> ETGASYITPYVPMPCMINDTHFLLRGPFEASWAIKLEITDVTTLVVDTDNVANPTNISKCFANNQDERLLGFTMEWFLSGLEHDHHFTPQIICGNVSKGEVNAQVNITMEDHCSQVFLKMRRIFGVFKNPCTSHGKQNVLISVSNWTNQCSGNHLSGTKHHHHHH

The GP1 subunit of the envelope-displayed arenaviral glycoprotein spike complex (GPC) mediates host cell recognition and is an important determinant of cross-species transmission. Maturation of the GPC precursor involves proteolytic cleavage of the polyprotein into a retained and myristoylated stable signal peptide (SSP), a GP1 attachment glycoprotein, and a membrane-anchored GP2 fusion glycoprotein (1–5). We solved the crystal structures of the GP1 glycoproteins from Loei River virus (LORV), an Asiatic rodent-borne OW arenavirus of unknown pathogenicity in humans, and Whitewater Arroyo virus (WWAV), an NW arenavirus associated with spillover into human populations in North America. Both WWAV and LORV GP1s were solved at neutral pH (7.5 to 8.0) and acidic pH (5.6 to 5.0), permitting the first direct analysis of the effect of pH on the structure of GP1 in the absence of cognate GP2.

Crystals of WWAV GP1 were generated under two conditions, buffered to pH 7.5 and 5.6, and X-ray diffraction data were collected to 2.4- and 2.0-Å resolution, respectively. As phase determination by molecular replacement with existing arenaviral GP1 structures failed to yield a solution, the single-wavelength anomalous-dispersion (SAD) method was used for structure elucidation. Crystallographic analysis of WWAV GP1 revealed the characteristic α/β fold that has been observed for other NW arenavirus GP1 structures, as well as in OW arenaviral GP1 glycoproteins in GP2-associated states, comprising a seven-stranded β-sheet with three α-helices positioned on the convex side of the molecule. WWAV GP1 structures determined at both neutral and acidic pHs are nearly identical (0.4-Å root mean square deviation [RMSD]), indicating that exposure to acidic endosomal pH, and subsequent shedding of GP1 from the GPC, is unlikely to induce conformational rearrangements to the molecule. Overlay analysis revealed that while the independently reported WWAV GP1 structures were essentially identical and exhibited an RMSD of 0.9 Å, minor structural differences were observed in loop 5 of the glycoprotein, indicating inherent flexibility in the region or a requirement for the quaternary architecture of the GPC for stabilization. Despite utilizing a common receptor, WWAV exhibits a low level of sequence conservation with other NW arenaviral GP1 glycoproteins with known structures (e.g., 24% and 25% identity to clade B JUNV and MACV, respectively), reflective of its classification as a clade D NW arenavirus. Consistent with a low level of sequence conservation with JUNV and MACV, WWAV GP1 exhibits significant structural variation throughout the α/β fold (2.3- to 2.5-Å RMSD). Comparison of our WWAV GP1 with other NW arenaviral GP1 structures revealed that while the NW arenaviral GP1 scaffold is structurally diverse, especially in loop regions, it adopts a single conformation that is independent of pH or the presence of ligand.> ELYPLTS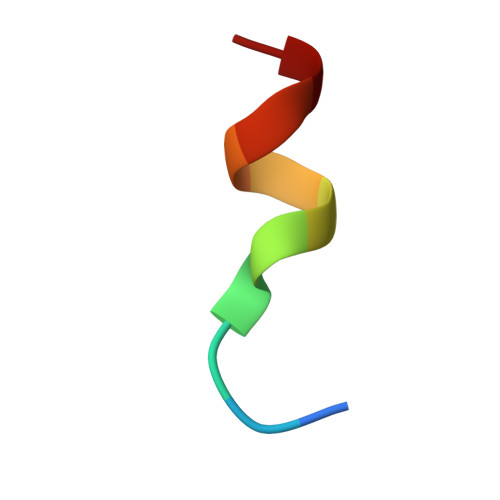LRSL>AERENLKNEATKVLEHVCEDINKESYGFVKISKMKENEKEIRLFNLEEIYHSLMKVGGSGATDGGKREDDAASHSVVAESNGAHLLQSDIWVRGRI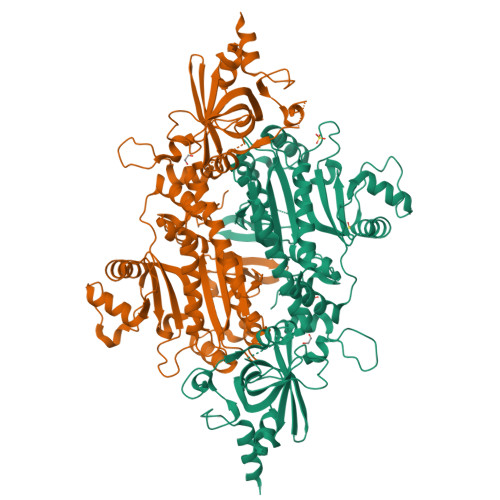HDIRSKGSLAFIILRHKLYSMQCILDIKHNDNDKNMMKWVSNLPLESIVDIKGKLSKPEVPIDSTNIKYEAHIRKIFCISKTAKELPFLLKDANMKETNEEGSIKVNQDNRLNNRCVDLRTYANYSIFCLQSQICTIFKNFLLENNFIEIHTPKLLGESSEGGANAFQINYFNQKGFLAQSPQLYKQMCINSGFDRVFEVAPVFRAENSNTYRHLCEYVSLDVEMTYKYDYLENVHFYDSMFKHIFTELSKGGKNEMLIKTVKGQYPCEDFQWLEETPIFTYEEAIKMLIQHGKLHLKEEEILAYDMSTDMEKELGKIVKASHHTDYYIIINFPSALRPFYTMYKEDEPAISNSYDFFMRGEEILSGSQRISDVNLLLENIKRFNLDANKLNFYIDSFAYSSYPHSGCGIGLERVLMLFLGLNNIRKTSLFPRDPKRLIP[2x]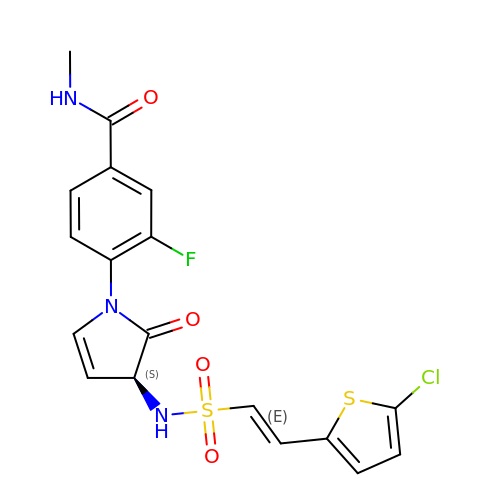4-[(3S)-3-({[(E)-2-(5-chlorothiophen-2-yl)ethenyl]sulfonyl}amino)-2-oxo-2,3-dihydro-1H-pyrrol-1-yl]-3-fluoro-N-methylbenzamide | C18 H15 Cl F N3 O4 S2 | AJYGFYXIRNIYPA-KGXGESDWSA-N> MLTMKDIIRDGHPTLRQKAAELELPLTKEEKETLIAMREFLVNSQDEEIAKRYGLRSGVGLAAPQINISKRMIAVLIPDDGSGKSYDYMLVNPKIVSHSVQEAYLPTGEGCLSV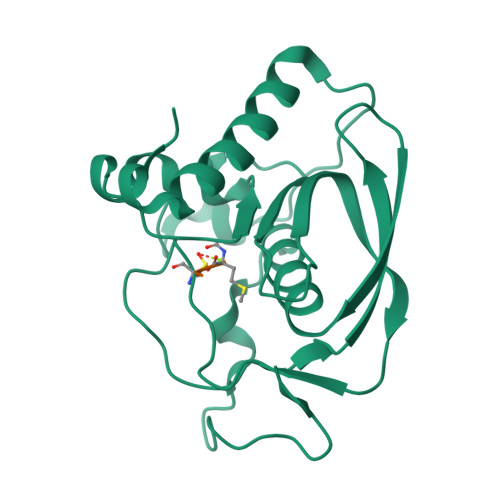DDNVAGLVHRHNRITIKAKDIEGNDIQLRLKGYPAIVFQHEIDHLNGVMFYDHIDKNHPLQPHTDAVEV;> MAS>AQPTNFHDQLKFAWLAGFVDADGCINAQIVSREDYLLKYQVRVSLTVFQSTTQHFILLDIQKILGCGTVRKRNDGMSEFCVVGGTSLQTTLEKLLPYLNLKRAQAKLVLQIIKKLPNTKDPSVLMEAALLADKVGLLTDGKKRTILAENVRECLKKLGHVVSAALEHHHHH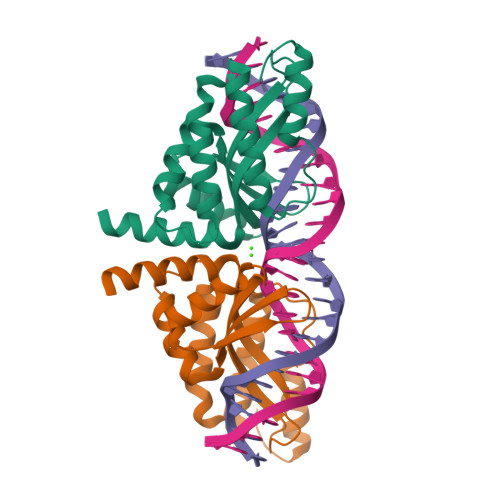H[2x]> MHHHHHHSSGRENLYFQGDDEIVHFSWKKGMLLNNAFLVIRKMGDGTFGRVLLCQHIDNKKYYAVKVVRNIKKYTRSAKIEADILKKIQNDDINNNNIVKYHGKFMYYDHMCLIFEPLGPSLYEIITRNNYNGFHIEDIKLYCIEILKALNYLRKMSLTHTDLKPENILLDDPYFEKSLITVRRVTDGKKIQIYRTKSTGIKLIDFGCATFKSDYHGSIINTRQYRAPEVILNLGWDVSSDMWSFGCVLAELYTGSLLFRTHEHMEHLAMMESIIQPIPKNMLYEATKTNGSKYVNKD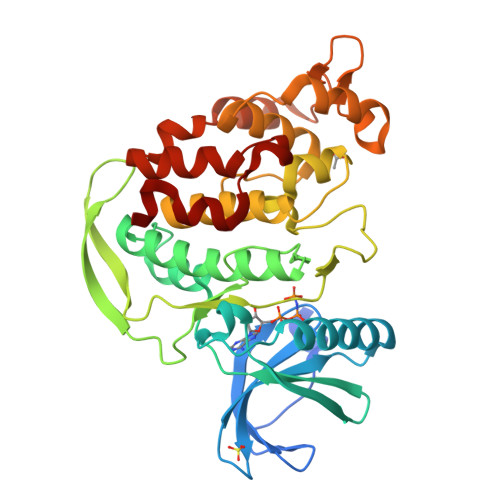ELKLAWPENASSINSIKHVKKCLPLYKIIKHELFCDFLYSILQIDPTLRPSPAELLKHKFLE>[3x]MTSLFEPAQAGDIALANRIVMAPLTRNRSPGAIPNNLNATYYEQRATAGLIVTEGTPISQQGQGYADVPGLYKREAIEGWKKITDGVHSAGGKIVAQIWHVGRISHTSLQPHGGQPVAPSAITAKSKTYIINDDGTGAFAETSEPRALTIDDIGLILEDYRSGARAALEAGFDGVEIHAANGYLIEQFLKSSTNQRTDDYGGSIENRARFLLEVVDAVAEEIGAGRTGIRLSPVTPANDIFEADPQPLYNYVVEQLGKRNLAFIHVVEGATGGPRDFKQGDKPFDYASFKAAYRNAGGKGLWIANNGYDRQSAIEAVESGKVDAVAFGKAFIANPDLVRRLKNDAPLNAPNQPTFYGGGAEGYTDYPALAQHHHHHH

We determined the crystal structure of the enzyme NerA, which has been shown to exhibit dual ene-reductase and nitro-reductase activity with α,β-unsaturated nitro compounds, from A. radiobacter. NerA exhibits a TIM-barrel fold typical for OYE-like proteins, and all catalytically important active site residues are conserved. Residues stabilizing the electron-withdrawing group (EWG; e.g., carbonyl, carboxylic acid, nitro) of a ligand in an ene-reductase-like reaction are a histidine/asparagine pair (H178 and N181). The putative proton donor residue is Y183.

Three enzyme molecules were present in the asymmetric unit, and the final model could be refined to R and Rfree values of 15.8 and 18.9 %, respectively. Structural superposition of the three monomers in the asymmetric unit gave very low RMSD values (Cα-RMSD for 371 aligned residues) of 0.160 Å for the superposition of chain A and chain B, 0.097 Å for that of chain A and chain C, and 0.216 Å for that of chain B and chain C. Larger structural differences are found in the regions of loop β3. In contrast, loop β3 in NerA is very long and forms a small subdomain. Loops of comparable length have only been described for two other OYE like proteins—PETNR from E. cloacae and SYE-1 from Shewanella oneidensis. Similarly to these two structures, NerA exhibits the highest crystallographic B factors in this capping subdomain. In the case of NerA, these residues are Y65 and Y356, and the geometric centers of their phenyl rings are 7.8 Å apart from each other. This distance places NerA in the “intermediate distance cluster” of OYEs. The experimentally determined moderate stereoselectivity of NerA with 1-nitro-2-phenylpropene (54 % ee for the reduced S-configured product)34 is in line with this prediction. For NerA we found that the biggest part of its active site is hydrophilic, with only a small hydrophobic patch located between the residues Y65 and Y356. In addition, a relatively hydrophobic region can be found parallel to the isoalloxazine ring of FMN; this indicates favorable binding of the substrate's aromatic/hydrophobic part in an orientation that results in a C=C double bond reduction.>[3x]MIHLYDAKSFAKLRAAQYAAFHTDAPGSWFDHTSGVLESVEDGTPVLAIGVESGDAIVFDKNAQRIVAYKEKSVKAEDGSVSVVQVENGFMKQGHRGWLVDLTGELVGCSPVVAEFGGHRYASGMVIVTGKGNSGKTPLVHALGEALGGKDKYATVRFGEPLSGYNTDFNVFVDDIARAMLQHRVIVIDSLKNVIGAAGGNTTSGGISRGAFDLLSDIGAMAASRGCVVIASLNPTSNDDKIVELVKEASRSNSTSLVISTDVDGEWQVLTRTGEGLQRLTHTLQTSYGEHAVLTIHTSKQSGGKQASGKAIQTVIKNDELESVLRRLTSN

The lipid-enveloped bacteriophages of the Cystoviridae family infect Gram-negative bacteria, mainly plant-pathogenic Pseudomonas species and share similarities with the members of the Reoviridae family, including bluetongue virus and rotavirus. Their genome of ∼14 kb consists of three dsRNA segments small (S), medium (M) and large (L), which are sequentially encapsidated as ssRNA precursors into the icosahedrally symmetric procapsid by the packaging NTPase P4 (15–23). P4 is a protein of ∼35 kDa, which can assemble into a hexameric ring. NTP-binding sites are located on the external perimeter of the ring at the interfaces between adjacent subunits, whereas the nucleic acid binding sites are found in the central channel. P4 proteins are the only known RNA-specific helicases belonging to helicase Superfamily 4 (SF4).

To understand this catalytic mechanism in detail, we performed side-directed mutagenesis of the residues in ɸ12 P4 involved in binding the nucleotide ring and analysed the mutants structurally and biochemically. In P4 ɸ12, the strand following the arginine finger motifs extends back into the ATP-binding site contributing two residues (Y288 and S292), which help position the nucleotide ring (see later in the text). A specific feature in ɸ12 P4 is a hydrogen bond between the hydroxyl of S292 and N7 of the purine ring. The substitution S292A did not prevent ATP binding but completely abolished ATPase activity owing to misplacement of the triphosphate moiety in the active site. Hence, purine specificity is achieved by locking the base by hydrogen bonding to the N7 site of a purine. The correct coordination of the base results in the precise alignment of the nucleotide that is essential for catalysis so that UTP is misaligned and not hydrolysed.>GHMGKVTKNSSSIKVVKLLVRLSDSVGYLFWDSATTGYATCFVFKGLFILTCRHVIDSIVGDGIEPSKWATIIGQCVRVTFGYEELKDKETNYFFVEPWFEIHNEELDYAVLKLKENGQQVPMELYNGITPVPLSG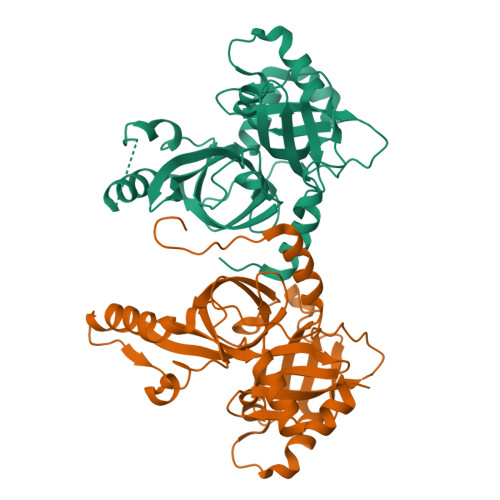LIHIIGHPYGEKKQIDACAVIPQGQRAKKCQERVQSKKAESPEYVHMYTQRSFQKIVHNPDVITYDTEFFFGAAGSPVFDSKGSLVAMHAAGFAYTYQNETRSIIEFGSTMESILLDIKQRHKPWYEEVFVNQQDVEMMSDEDL[4x]> 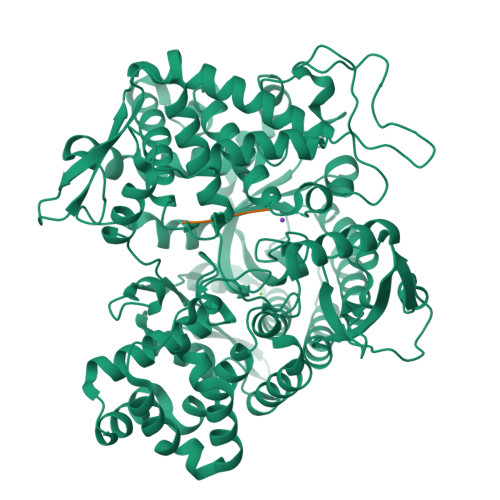MADTQYILPNDIGVSSLDCREAFRLLSPTERLYAYHLSRAAWYGGLAVLLQTSPEAPYIYALLSRLFRAQDPDQLRQHALAEGLTEEEYQAFLVYAAGVYSNMGNYKSFGDTKFVPNLPKEKLERVILGSEAAQQHPEEVRGLWQTCGELMFSLEPRLRHLGLGKEGITTYFSGNCTMEDAKLAQDFLDSQNLSAYNTRLFKEVDGEGKPYYEVRLASVLGSEPSLDSEVTSKLKSYEFRGSPFQVTRGDYAPILQKVVEQLEKAKAYAANSHQGQMLAQYIESFTQGSIEAHKRGSRFWIQDKGPIVESYIGFIESYRDPFGSRGEFEGFVAVVNKAMSAKFERLVASAEQLLKELPWPPTFEKDKFLTPDFTSLDVLTFAGSGIPAGINIPNYDDLRQTEGFKNVSLGNVLAVAYATQREKLTFLEEDDKDLYILWKGPSFDVQVGLHALLGHGSGKLFVQDEKGAFNFDQETVINPETGEQIQSWYRSGETWDSKFSTIASSYEECRAESVGLYLCLHPQVLEIFGFEGADAEDVIYVNWLNMVRAGLLALEFYTPEAFNWRQAHMQARFVILRVLLEAGEGLVTITPTTGSDGRPDARVRLDRSKIRSVGKPALERFLRRLQVLKSTGDVAGGRALYEGYATVTDAPPECFLTLRDTVLLRKESRKLIVQPNTRLEGSDVQLLEYEASAAGLIRSFSERFPEDGPELEEILTQLATADARFWKGPSEAPSGQA> MEKMSRVTTALGGSVLTGRTMHCHLDAPANAISVCRDAAQVVVAGRSIFKIYAIEEEQFVEKLNLRVGRKPSLNLSCADVVWHQMDENLLATAATNGVVVTWNLGRPSRNKQDQLFTEHKRTVNKVCFHPTEAHVLLSGSQDGFMKCFDLRRKDSVSTFSGQSESVRDVQFSIRDYFTFASTFENGNVQLWDIRRPDRCERMFTAHNGPVFCCDWHPEDRGWLATGGRDKMVKVWDMTTHRAKEMHCVQTIASVARVKWRPECRHHLATCSMMVDHNIYVWDVRRPFVPAAMFEEHRDVTTGIAWRHPHDPSFLLSGSKDSSLCQHLFRDASQPVERANPEGLCYGLFGDLAFAAKESLVAAESGRKPYTGDRRHPIFFKRKLDPAEPFAGLASSALSVFETEPGGGGMRWFVDTAERYALAGRPLAELCDHNAKVARELGRNQVAQTWTMLRIIYCSPGLVPTANLNHSVGKGGSCGLPLMNSFNLKDMAPGLGS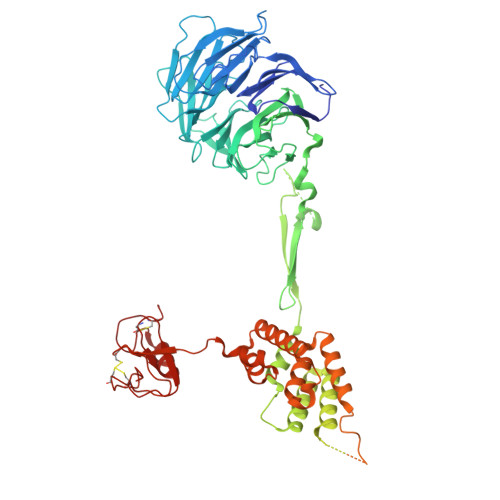ETRLDRSKGDARSDTVLLDSSATLITNEDNEETEGSDVPADYLLGDVEGEEDELYLLDPEHAHPEDPECVLPQEAFPLRHEIVDTPPGPEHLQDKADSPHVSGSEADVASLAPVDSSFSLLSVSHALYDSRLPPDFFGVLVRDMLHFYAEQGDVQMAVSVLIVLGERVRKDIDEQTQEHWYTSYIDLLQRFRLWNVSNEVVKLSTSRAVSCLNQASTTLHVNCSHCKRPMSSRGWVCDRCHRCASMCAVCHHVVKGLFVWCQGCSHGGHLQHIMKWLEGSSHCPAGCGHLCEYS We present two cases of protein structures determined by As-SAD phasing in our laboratory during the last two years, a putative PncA from Streptococcus mutans and caspase-6 from Homo sapiens. The crystallization conditions of both proteins contained cacodylate buffer, which specifically modified surface cysteines of the proteins. Both datasets were collected on SR facilities at the wavelength of 1.000 Å, the high-energy end from the K absorption edge of As (∼ 1.04 Å), and sufficient anomalous signals for SAD phasing were obtained. Our current studies demonstrated that cacodylate buffer is an effective reagent to covalently modify protein surface cysteines, and that As could serve as an ideal anomalous scatterer in SAD phasing method.

In both SmPncA and Casp6, arsenic atoms were incorporated into proteins by chemical reaction between cysteines and cacodylic acid. In the case of Casp6, proteins were prepared with DTT to avoid the formation of disulfide bond between free cysteines. When protein solution containing DTT was mixed with the crystallization reservoir, cacodylic acid was spontaneously reduced to a chemically more active As (III)-thiolate intermediate. The As (III) reagent in turn reacted with cysteines by a thiol exchange process, resulting in the formation of a cacodyl-cysteine product. In this case, four out of ten cysteines in the protein covalently bound to As, while the other six cysteines were either solvent inaccessible or occupied by the inhibitor Ac-VEID-CHO in the active site.

>AFYKREMFDPAEKYKMDHRRRGIALIFNHERFFWHLTLPERRGTCADRDNLTRRFSDLGFEVKCFNDLKAEELLLKIHEVSTVSHADADCFVCVFLSHGEGNHIYAYDAKIEIQTLTGLFKGDKCHSLVGKPKIFIIQACRGNQHDVPVIPLDVVDNQTEKLDTNITEVDAASVYTLPAGADFLMCYSVAEGYYSHRETVNGSWYIQDLCEMLGKYGSSLEFTELLTLVNRKVSQRRVDFCKDPSAIGKKQVPCFASMLTKKLHFFPKSNLEHHHHHH[2x];>[2x]XVEID3-[5-(aminomethyl)-4-(carboxymethyl)-2-iodo-1H-pyrrol-3-yl]propanoic 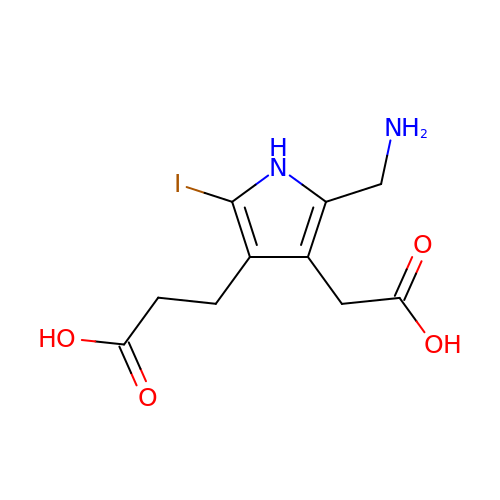acid | C10 H13 I N2 O4 | SQCPKOTYDSJOKL-UHFFFAOYSA-N>[4x]MKVWLVGAYGIVSTTAMVGARAIERGIAPKIGLVSEL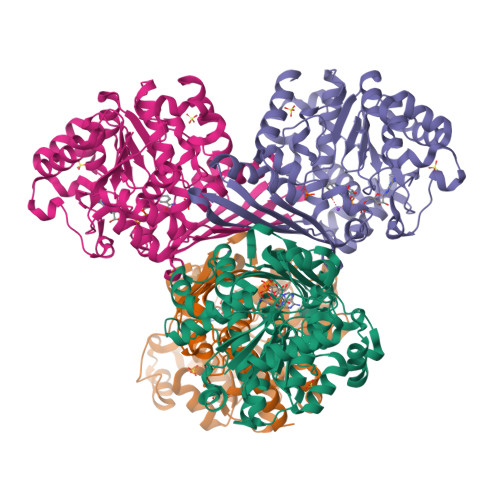PHFEGIEKYAPFSFEFGGHEIRLLSNAYEAAKEHWELNRHFDREILEAVKSDLEGIVARKGTALNCGSGIKELGDIKTLEGEGLSLAEMVSRIEEDIKSFADDETVVINVASTEPLPNYSEEYHGSLEGFERMIDEDRKEYASASMLYAYAALKLGLPYANFTPSPGSAIPALKELAEKKGVPHAGNDGKTGETLVKTTLAPMFAYRNMEVVGWMSYAILGDYDGKVLSARDNKESKVLSKDKVLEKMLGYSPYSITEIQYFPSLVDNKTAFDFVHFKGFLGKLMKFYFIWDAIDAIVAAPLILDIARFLLFAKKKGVKGVVKEMAFFFKSPMDTNVINTHEQFVVLKEWYSNLK> AVPSTQTPWGIKSIYNDQSITKTTGGSGIKVAVLDTGVYTSHLDLAGSAEQCKDFTQSNPLVDGSCTDRQGHGTHVAGTVLAHGGSNGQGVYGVAPQAKLWAYKVLGDNGSGYSDDIAAAIRHVADEASRTGSKVVINMSLGSSAKDSLIASAVDYAYGKGVLIVAAAGNSGSGSNTIGFPGGLVNAVAVAALENVQQNGTYRVADFSSRGNPATAGDYIIQERDIEVSAPGASVESTWYTGGYNTISGTSMATPHVAGLAAKIWSANTSLSHSQLRTELQNRAKVYD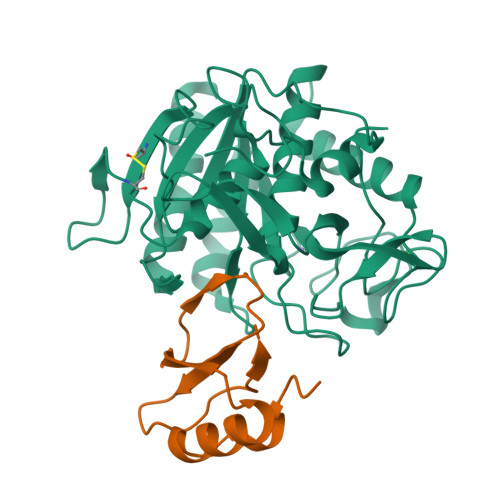IKGGIGAGTGDDYASGFGYPRVK;> TGAGDRHNLKTEWPELVGKSVEEAKKVILQDKPEAQIIVLPVGTIVTMEYRIDRVRLFVDKLDNIAQVPRVG>[2x]MALAKRIDAALIVKDGRVVEGSNFENLRDSGDPVELGKFYSEIGIDELSFWDITASVEKRKT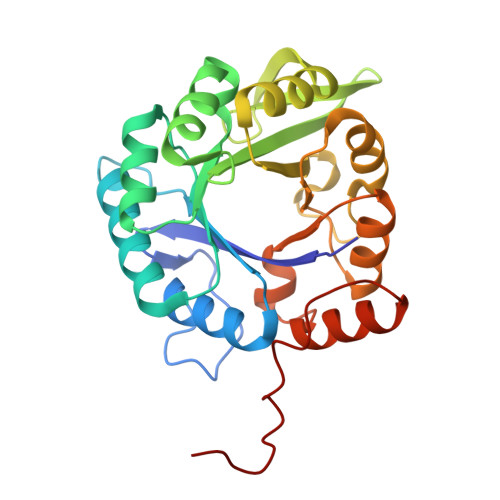MLELVEKVAEQIDIPFTVGGGIHDFETASELILRGADKVEINTAAVENPSLITQIAQTFGSQAVVVYIAAKRVDGEFMVFTYSGTKNTGILLRDWVVEVEKRGAGEIVLGSIDRLGTKSGYDTEMIRFVRPLTTLPIIAHRGAGKMEHFLEAFLAGADAAKADSVFHFREIDVRELKEYLKKHGVNVRLEGLGSLEHHHHHH> IPVIEPLFTKVTEDIPGAEGPVFDKNGDFYIVAPEVEVNGKPAGEILRIDLKTGKKTVICKPEVNGYGGIPAGCQCDRDANQLFVADMRLGLLVV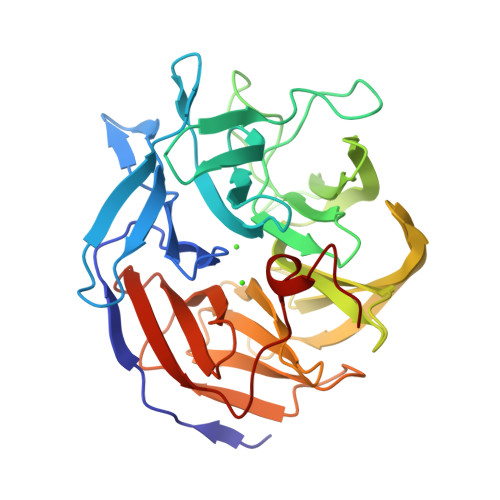QTDGTFEEIAKKDSEGRRMQGCNDCAFDYEGNLWITAPAGEVAPADYTRSMQEKFGSIYCFTTDGQMIQVDTAFQFPNGIAVRHMNDGRPYQLIVAETPTKKLWSYDIKGPAKIENKKVWGHIPGTHEGGADGMDFDEDNNLLVANHGSSHIEVFGPDGGQPKMRIRCPFEKPSNLHFKPQTKTIFVTEHENNAVWKFEWQRNGKKQYCETLKFGIF>SETSRTAFGGRRAVPPNNSNAAEDDLPTVELQGVVPRGVNLQEFLNVTSVHLFKERWDTNKVDHHTDKYENNKLIVRRGQSFYVQIDFSRPYDPRRDLFRVEYVIGRYPQENKGTYIPVPIVSELQSGKWGAKIVMREDRSVRLSIQSSPKCIVGKFRMYVAVWTPYGVLRTSRNPETDTYILFNPWCEDDAVYLDNEKEREEYVLNDIGVIFYGEVNDIKTRSWSYGQFEDGILDTCLYVMDRAQMDLSGRGNPIKVSRVGSAMVNAKDDEGVLVGSWDNIYAYGVPPSAWTGSVDILLEYRSSENPVRYGQCWVFAGVFNTFLRCLGIPARIVTNYFSAHDNDANLQMDIFLEEDGNVNSKLTKDSVWNYHCWNEAWMTRPDLPVGFGGWQAVDSTPQENSDGMYRCGPASVQAIKHGHVCFQFDAPFVFAEVNSDLIYITAKKDGTHVVENVDATHIGKLIVTKQIGGDGMMDITDTYKFQEGQEEERLALETALMYGAKKPLNTEGVMKSRSNVDMDFEVENAVLGKDFKLSITFRNNSHNRYTITAYLSANITFYTGVPKAEFKKETFDVTLEPLSFKKEAVLIQAGEYMGQLLEQASLHFFVTARINETRDVLAKQKSTVLTIPE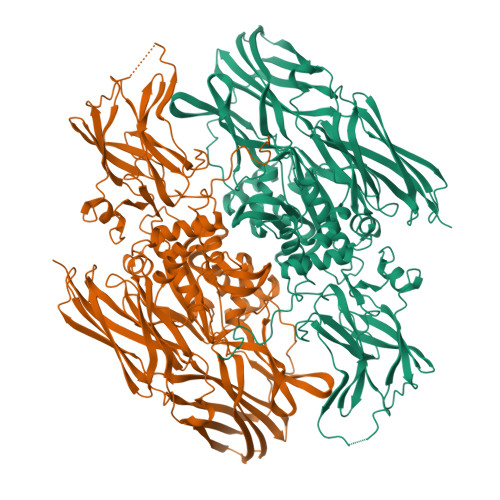IIIKVRGTQVVGSDMTVTVEFTNPLKETLRNVWVHLDGPGVTRPMKKMFREIRPNSTVQWEEVCRPWVSGHRKLIASMSSDSLRHVYGELDVQIQRRPSM[2x]>[2x]NQPDWADEAANGAHQDAWKSLKADVENVYYMVKATYKNDPVWGNDFTCVGVMANDVNEDEKSIQAEFLFMNNADTNMQFATEKVTAVKMYGYNRENAFRYETEDGQVFTDVIAYSDDNCD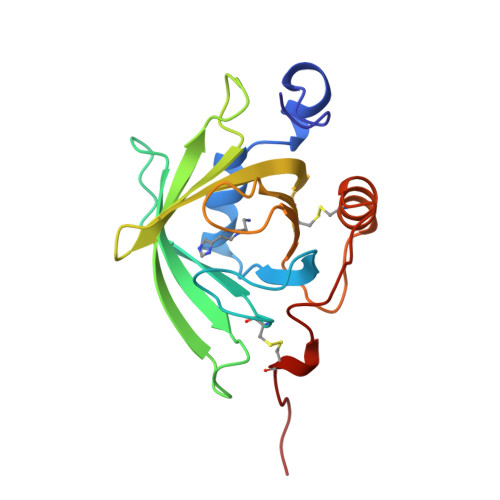VIYVPGTDGNEEGYELWTTDYDNIPANCLNKFNEYAVGRETRDVFTSACLEIAAA> MFENITTAPADPILGLADLLRADERPGKIDLGMGVYNDETGKTPVLTSVKKAEQYLLENETTKNYLGIDGIPEFGRCTQELLFGKGSALINDKRARTAQTPGGTGALRVAADFLAKNTSVRRVWVSNPGWPTHKSVFNSAGLEVREYAYYDAENHTLDFDALINSLNEAQAGDVVLFHGCCHNPTGIDPTLEQWQTLAQLSVEKGWLPLFDFAYQGFARGLEEDAEGLRAFAAMHKE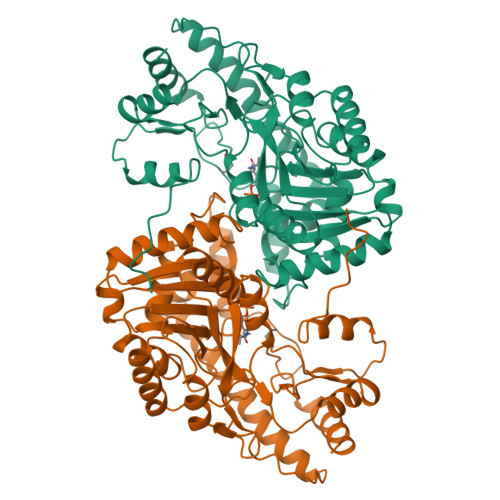LIVASSYSKNFGLYNERVGTCTLVAADSETVDRAFSQMKAAIRVNYSSPPAHGASVVATILGNDALRAIWEQELTDMRQRIQRMRQLFVNTLQEKGANRDFSFTIKQNGMFFFGGLTKEQVLRLREEFGVYAVASGRLNVAGMTPDNLAPLCEAIVAVL> GMGDAPSPEEKLHLITRNLQEVLGEEKLKEILKERELKIYWGTATTGKPHVAYFVPMSKIADFLKAGCEVTILFADLHAYLDNMKAPWELLELRVSYYENVIKAMLESIGVPLEKLKFIKGTDYQLSKEYTLDVYRLSSVVTQHDSKKAGAEVVKQVEHPLLSGLLYPGLQALDEEYLKVDAQFGGIDQRKIFTFAEKYLPALGYSKRVHLMNPMVPGLTGSKMSSSEEESKIDLLDRKEDVKKKLKKAFCEPGNVENNGVLSFIKHVLFPLKSEFVILRDEKWGGNKTYTAYVDLEKDFAAEVVHPGDLKNSVEVALNKLLDPIREKFNTPALKKLASAAYPDPSKQKPMAKGPAKNSEPEEVI

Like E1 enzymes, aminoacyl tRNA synthetases (aaRSs) are adenylate-forming enzymes (AFEs). They catalyze the transformation of amino acids into AMP conjugates, and then into aminoacyl-tRNAs, to supply protein synthesis. PfYRS is a Class I aaRS, characterized by a catalytic domain that adopts a Rossmann fold (residues 18–260) linked to a C-terminal domain (residues 261–370) that is involved in recognition of the anticodon stem of tRNATyr. PfYRS contains the two motifs characteristic of the catalytic domain of Class I (sub-class c) tRNA synthetases: “HIGH” and “KMSKS” (70HIAQ73 and 247KMSKS251 in PfYRS).

X-ray crystallographic studies of plasmodium and human YRSs reveal differential flexibility of a loop over the catalytic site that underpins differential susceptibility to reaction-hijacking by ML901. Importantly, recombinant HsYRS was not stabilized in the presence of ML901 plus substrates, suggesting the inhibitory species is not produced by, or does not bind to, the human enzyme (red curves). Similarly, ML901 inhibits tRNATyr acylation to tyrosine in vitro by PfYRS, but not by HsYRS. We were not able to generate a structure of HsYRS in complex with enzyme-generated ML901-Tyr as HsYRS does not catalyze formation of the conjugate. S15F), the 222KMSSS226 loops were not defined in the electron density (Fig. 5Cii; fig. That is, the decreased susceptibility of HsYRS and PfYRSS234C to reaction hijacking by ML901 is associated with mobility of the KMSSS/KMSKS loop, which is, in turn, associated with rotation of the His49/70 side chain. These conformational changes may promote dissociation of the charged tRNA, thereby preventing the hijacking reaction.We recently identified an atypical bifunctional dioxygenase CcTet from Coprinopsis cinerea that works on both 5mC and 6mA demethylation. We recently demonstrated that CcTet, which was previously identified as a C. cinerea 5mC dioxygenase, also functions as a dsDNA 6mA demethylase. Its catalysis not only of conventional 5mC oxidation during the DNA active demethylation process, but also of dsDNA 6mA demethylation makes it a bifunctional dsDNA demethylase. In complex with dsDNA, the middle of the enzyme contained two anti-parallel β-sheet layers comprising 12 β-strands total, with one sheet containing β6-β11-β8-β9 and the other containing β4-β5-β12-β7-β10-β3-β2-β1. These sheets formed a jelly-roll catalytic pocket to accommodate cofactors and substrates.

The complex of CcTet-Δ16 and 12-bp 5mC-dsDNA oligo was crystallized at 277 K in the presence of manganese(II) (Mn2+) and a catalytically inactive analog of 2-oxoglutarate, NOG. The resolved structure suggested that there were four CcTet–5mC-dsDNA complexes in each asymmetric unit. Loop1 and loop3 inserted into the dsDNA minor groove, whereas the α′/loop′ region bound to the edges of the dsDNA strands near the major groove. Unexpectedly, the dsDNA strands in the CcTet–5mC-dsDNA complex were rotated ∼5° anticlockwise due to compression by the loop1 and α′/loop′ regions; this indicated an alternative mode of 5mC-dsDNA binding compared to 6mA-dsDNA. Instead, Arg92 and Arg96 formed salt bridge interactions with the O2 atoms of dT4 and dC5, or with the backbone phosphate of dC5, pushing the dsDNA strands outward by ∼3.6 Å compared to the 6mA-dsDNA bound form. Specifically, in the CcTet–5mC-dsDNA complex, the finger residue Val232 was stacked between dC5 and dG7 through hydrophobic interactions; the stacked residue then pushed the 5mC base, causing it to flip into the active pocket for subsequent catalysis. The cofactors Mn2+ and NOG and the flipped 5mC substrate were stabilized in the correct positions and orientations inside the active pocket through multiple hydrophobic and hydrophilic interactions. Mn2+ was primarily stabilized via octahedral coordinate interactions with the side chains of His326, His376 and Asp328, a water molecule, and the NOG C5-carboxyl and C4-ketone groups. Specifically, the 5mC base was stacked between Phe391 and Arg205, which were conserved among the family members, with the exception of a Tyr in place of the Phe in hTet2. In contrast, the Asp337 side chain rotated ∼90° in complex with 5mC-dsDNA to form two indirect hydrophilic interactions (through two water molecules) with the N4 atom of the 5mC pyrimidine ring, further stabilizing the 5mC base inside the active pocket.

>[4x]MSAIPFSTDDCSQDETLPSLLLIDEAAAVLGRMIQGLRTGIPYIHTENDSIKANPILRTALWQAAYVLEKAYRRRYRVPWTARRYMRELTPRQDGRNANREAVMAKEFPPGAELNSDHPVQEILPAMIIDAEDHILFCYLPSCVSPAIMTIIDAAVGTLATTKDGHLQKKSRAREGERARVEMQKVKGKGKQEEEGQEKLGANWREALDLFRQGACKMTPGVLTFAPAWWPVGHENQLPGPASTLKPPKGEGRMFLSDIPIASALVGAILAQINQPLFESGVKVLRELYSNSKLTKDHSTVSKIIEIWFSPFSSLSLIVNRATPIHRDTSGPIEGMDILVTGGNYSNGVLVTPSFNRRWTYNPGCVVALLGKLVLHGVPEVDGERYCMAHFWRERLFDAAGVPFPYPSKWQESYT> KETAAAKFERQHMDSSTSAASSSNYCNQMMKSRNLTKDRCKPVNTFVHESLADVQA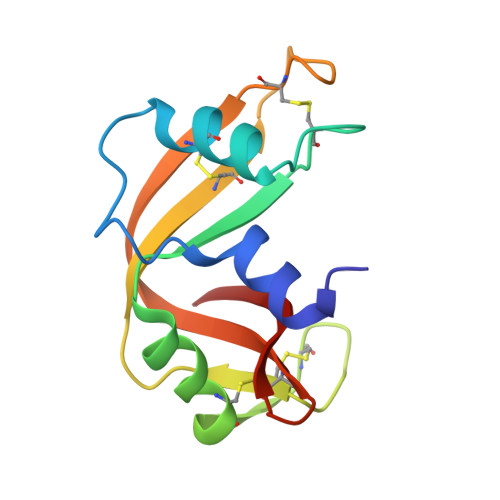VCSQKNVACKNGQTNCYQSYSTMSITDCRETGSSKAPNCAYKTTQANKHIIVACEGNPYVPVHFDASV>MELKSTRHTKYLCNYHFVWIPKHRRNTLVNEIAEYTKEVLKSIAEELGCEIIALEV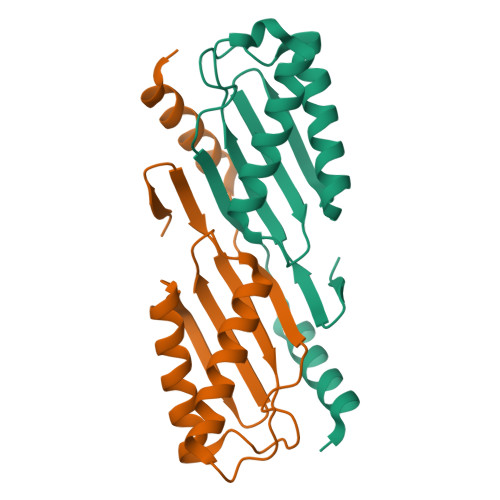MPDHIHLFVNCPPRYAPSYLANYFKGKSARLILKKFPQLNKGKLWTRSYFVATAGNVSSEVIKKYIEEQWRKEGEEE[2x]>SMNPIEDDLIFRVGTKGRNKGEFTNLQGVAASTNGKILIADSNNQCVQIFSNDGQFKSRFGIRGRSPGQLQRPTGVAVHPSGDIIIADYDNKWVSIFSSDGKFKTKIGSGKLMGPKGVSVDRNGHIIVVDNKACCVFIFQPNGKIVTRFGSRGNGDRQFAGPHFAAVNSNNEIIITDFHNHSVKVFNQEGEFMLKFGSNGEGNGQFNAPTGVAVDSNGNIIVADWGNSRIQVFDGSGSFLSYINTSADP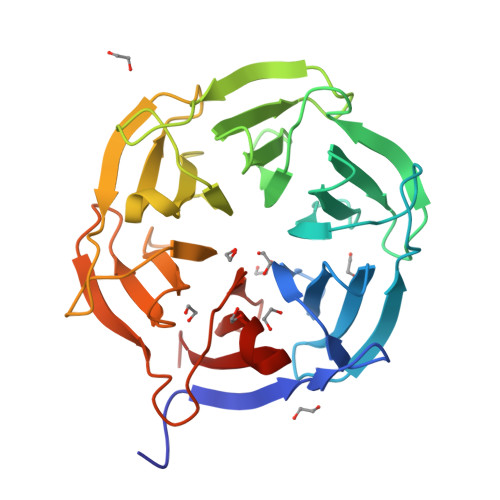LYGPQGLALTSDGHVVVADSGNHCFKVYRYLQ[4x]~{N}-(4-phenoxyphenyl)-7~{H}-pyrrolo[2,3-d]pyrimidin-4-amine 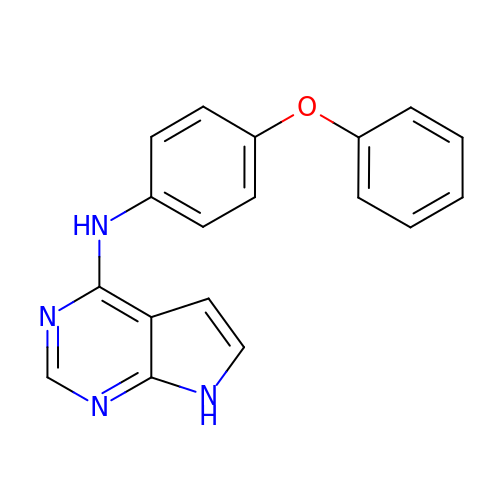| C18 H14 N4 O | QZBWRRCYSQGONG-UHFFFAOYSA-N2-fluoranyl-5-sulfo-benzoic acid | C7 H5 F O5 S | 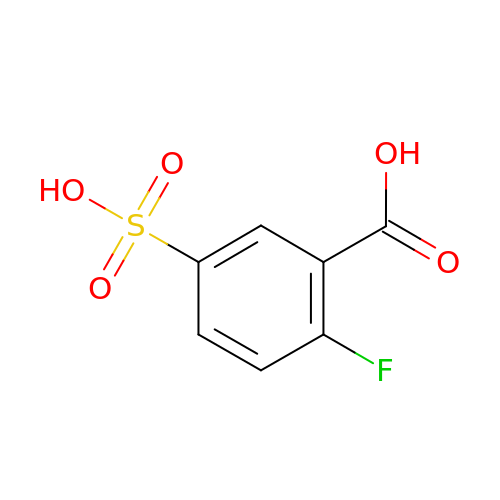DAYQUMDMVVFSIW-UHFFFAOYSA-N> GSHMTPQLLEEQERLIATLIEAHRKTYDASYSDFSQFRPPKRGDGSPECRNATNPFLMSLLNSDMDELPKASASGAEAAAGDELSMLPHLADLVSYSIQKVIGFAKMIPGFKELCTEDQISLLKASAIEIIILRSNESFTMEDNSWTCGSNEFKYQIGDVMQAGHKLELLEPLVKFQVNMKKLDLHEAEHVLL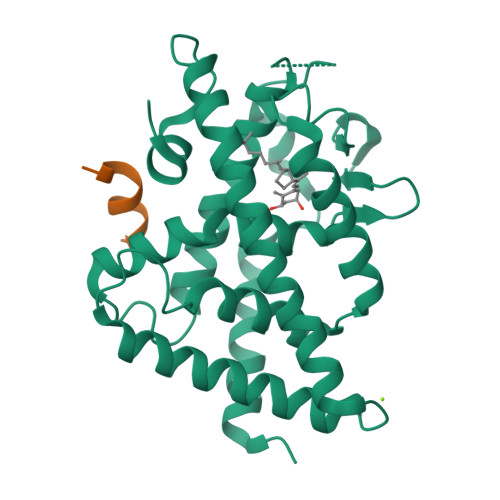MAICLFSPDRPGVQDRCRVEEVQEHLTETLRAYIACRHPLSCKHMLYTKMVEKLTELRSLNEEHSKQYLQISQDAVNKEDLPPLLLEVFGNPTA;> RHKILHRLLQEGS>QKGPVFLKEPTNRIDFSNSTGAEIECKASGNPMPEIIWIRSDGTAVGDVPGLRQISSDGKLVFPPFRAEDYRQEVHAQVYACLARNQFGSIISRDVHVRAVVIQSYESEADNEYVIRGNSVVMKCEIPSYVADFVFVDLWLDSEGRNYYPNNAAETDGKYLVLPSGELHIREVGPEDGYKSYQCRTKHRLTGETRLSATKGRLVITEPVGSVRPKVNPQDKHQFIDVELASSYSLLCMAQSYPTPSFRWYKFIEGTTRKQA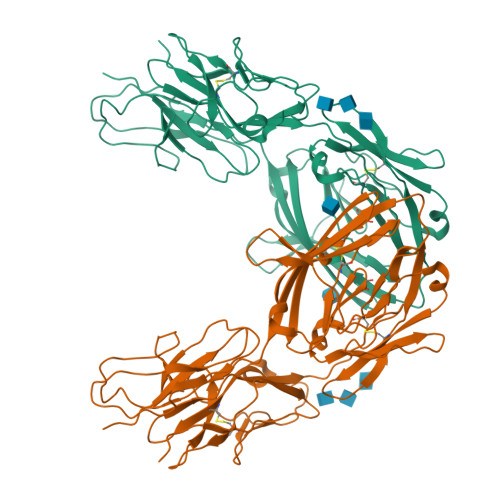VVLNDRVKQVSGTLIIKDAVVEDSGKYLCVVNNSVGGESVETVLTVTAPLSAKIDPPTQTVDFGRPAVFTCQYTGNPIKTVSWMKDGKAIGHSESVLRIESVKKEDKGMYQCFVRNDRESAEASAELKLG[2x]> MATRPTGFDKAKERAKQWLKDRFQRTDLFTCEPGAVDARTTSRIEKATRKLLTLCSNKRLKLKNSPPYLQGILFDTNDFFRRIFSLNTLDTLRDCPYLNLAVRKYLIHCRIATKLFRDAGEEMESEDSEYRRQLNKYTLVFSHMLADLQAVYKDGHLDADFTIVKIDAREF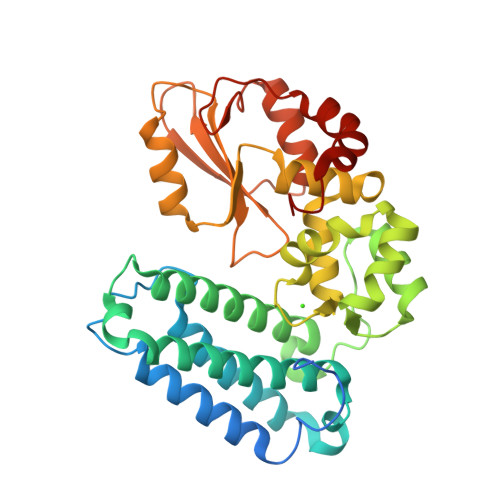WHRQFGKRLVVPWSELVPIMQAELGLSEKEGPALQHTMDITENNHVSWFEFDVFTRLFQPWSQLINNWYVLALNHPAYKAFITYDEVEAILRHHLHRPGSYVYRLSCTRLGQWAIGFVTRAGKIVQTIPQNKSLYQALLDGVEERLYLYPDGKNVQLDLKRMISDAPQNRVQVTKEEY Bin2 (also called BRAP1) is a putative membrane remodelling protein whose function is unknown but high levels of mRNA are found in leucocytes and leukaemic cells. The N-BAR domain of Bin2 is positioned within the BAR domain superfamily of membrane remodelling domains alongside the N-BAR domains of amphiphysins and endophilins. One such association occurs in a subgroup of BAR family members that have an additional N-terminal amphipathic helix which inserts in a shallow manner into the bilayer and induces positive curvature, that is consistent with, and stabilized by the BAR domain architecture. These N-BAR domains exert both intrinsic (amphipathic helix) and extrinsic forces (BAR module) on the membrane to promote changes in membrane curvature. Taken together, these data suggest that Bin2 is a bona fide member of the N-BAR protein family that has an important role in leucocyte morphogenesis.

The structure of the predicted Bin2 BAR was determined by MIRAS using a native crystal and a Se-Met derivative. A dimer was present in the asymmetric unit and the general architecture of the dimer resembled an elongated banana as found for other BAR modules. Each monomer was a coiled-coil, formed by three long, bent helices. Helix 1 comprised amino acids 38 to 88, helix 2 (from 95 to 159) was kinked in two places, at residues Asp119 and Gln131 (labelled as K1 and K2 in Figure 2A), and helix 3 (residues 169 to 238) was disrupted at Pro196 (K3 in Figure 2A). Different conformations for the extended regions of the dimer wings were observed for each monomer in the dimer. Concretely, the region between kinks K2 and K3 (amino acids 131 to 196) showed different conformations in each monomer and this was likely due to crystallographic contacts. The movement can be described as a lateral displacement of helices 2 and 3. This does not affect the curvature defined by the concave face of the dimer, which would be consistent with a scaffolding mechanism for membrane binding, where a defined membrane binding interface is needed. The overall fold of hBin2 BAR was very similar to that of Amph BAR consistent with the high sequence homology with dAmph and hAmph2 (N-BAR sequence identity of 37% and 62%, respectively). The concave face can accommodate a circle of diameter 170 Å, which was slightly smaller than that of Amph due to the way the protomers intersected and the distinct helix kinking. The dimerization interface of hBin2 was smaller than those of dAmph or hAmph2.

>GSKFSRAQEKVLQKLGKAVETKDERFEQSANNFYQQQAEGHKLYKDLKNFLSAVKVMHESSKRVSETLQEIYSSEWDGHEELKAIVWNNDLLWEDYEEKLADQAVRTMEIYVAQFSEIKERIAKRGRKLVDYDSARHHLEAVQNAKKKDEAKTAKAEEEFNKAQTVFEDLNQELLEELPILYNSRIGCYVTIFQNISNLRDVFYREMSKLNHNLYEVMSKL[2x]5-ethynyl-7-(beta-D-ribofuranosyl)-7H-pyrrolo[2,3-d]pyrimidin-4-amine 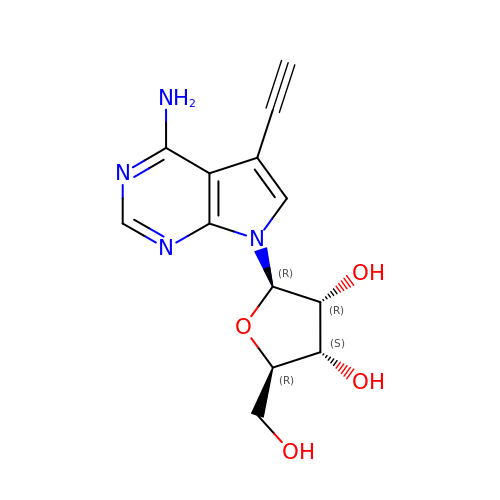| C13 H14 N4 O4 | ANCWCJFYCNNXDR-QYVSTXNMSA-N The CorA/Mrs2 family of pentameric proteins are cardinal for the influx of Mg2+ across cellular membranes, importing the cation to mitochondria in eukaryotes. The mitochondrial inner membrane protein Mrs2 (mitochondrial RNA-splicing protein 2) is responsible for regulating the Mg2+ concentrations of mitochondria in eukaryotes, providing controlled uptake of the ion14–16. CorA/Mrs2 forms homopentamers with two transmembrane (TM) helices (TM1 and TM2) in each monomer, which are preceded by a soluble N-terminal domain (NTD) that regulates the Mg2+ passage. The protein family exposes only the loop between TM1 and TM2 to the surrounding environment but this stretch harbors a conserved selective filter GMN motif that is essential for permeation.

We first maintained Mg2+ in all procedures during sample preparation. The final reconstructed map reached an average resolution of 3.1 Å in the absence of imposed symmetry. Finally, two additional features of the cryo-EM density in the pore are assigned as Mg2+ ions, the first located at T434 (glycine in hMrs2) and the second positioned at the conserved T427. Three more constriction regions of the pore follow P2, marked by D420 (asparagine in hMrs2), the conserved M417–R413 pair that is positioned at the membrane interface to the matrix and the R406 (phenylalanine in hMrs2)–D410 (invariant) pair. Nonetheless, the combination of invariant positively charged residues at R413 and a hydrophobic or positively charged lock for cations at R406, along with the small diameters at these constrictions (4.0 and 2.0 Å, respectively, representing the narrowest parts of the permeation pathway), indicates that the CtMrs2 structure is closed. The cryo-EM density reveals the presence of four more putative Mg2+-binding sites per monomer, present as a ‘glue’ in between separate polypeptides in the soluble fraction of CtMrs2. One pair of these sites (M1 and M2; M for the matrix of the mitochondria) are positioned at the tip of the protein. The second pair of putative Mg2+-binding sites (here denoted M3 and M4) are located in between the stalk helix of one monomer and helix α5 of the adjacent monomer. In the closed state, Mg2+ ions bind between the NTDs of separate monomers (positions M1 and M4 or M1–M4 in CtMrs2), thereby assisting in stabilizing the symmetrical shape, and to distinct positions of the pore (U, S, P1 and P2). At elevated Mg2+ concentrations in the matrix, Mrs2 is stabilized in a closed configuration through Mg2+ that bridges the monomers, two of which (sites M1 and M4) are conserved in Mrs2, including hMrs2.

>[5x]SGRLTWRELLFGSGARKQSEAMKEEEIMMRLQEDSGAIFQRRSLTSKAALDPRLRCTEVDGNGNVIMVDGELKKSELIAKYGLLPRDLRKIDSSNLPHILVRPSAILINLLHLKVLIKHDRVLLFDVYGSTSSYPQSAFMYDLQGKLQQKQTGGANSLPYEFRALEAVLMSVTAELEADFEAVRDPVIRILSELEDDIDREKLRILLVLSKRVSTFEQKAKLVRDAIEELLEADDDLAAMYLTEKTHDLYRGEDDHTEVELLLESYHKLCDEVVQEASNLVSSIRNTEEIIRAILDANRNSLMLLDLKFSIGTLGLAMGTFLAGLYGMNLENFIEETNWGFGAITGLSTLLSLVVCWYGLAKLRKVQRVKMNGAGFTRHNHWFRDDSTDVLLDPSNRERLRKINMMKSHAKQKTAAAKKWPLNKL>[2x]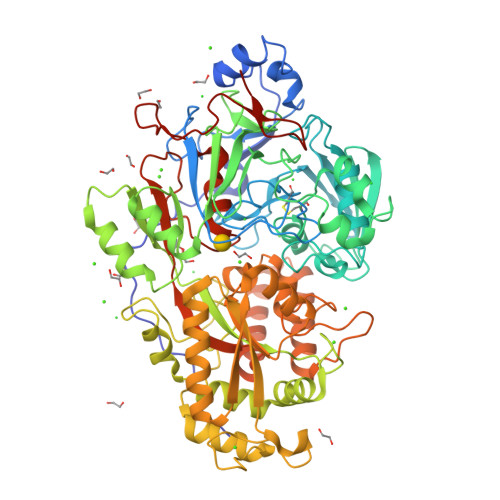MIALSANAFETTTPPEPPQFPAEGKINYVARDTILEFKALPSYSEPDWITEKFEKAGKLPPLKERLPEEPLVYKTGNMPDGVGVYGDTMRHVVGGRPEGWNYIAGQSQGWGGIDIALSECLTRTAPLFQVDAKDTEPLPNLAKSWEWSEDGHTLTMHLVKGAKWSDGEAFNADDVMFYWEDAVVDPNVSPLGGGASPEAFGEGTTLKKIDDYTVEWTFKAAFPKQYLYTMAYPSFCPGPSHILKPQHPKYSKNTYNQFKNAFPPEYMNMPVMGAWVPVSYRPDDLIVLRRNPYYWKVDEKGQQLPYLNEVHYKLSTWADRDVQAVAGSGDFSNLEQPENFVASLKRAADPNAPARLAFGPRLIGYNLQMNFSANGWGNPDERGQAIRELNRNEVFRQAVTSALDRKAIGDSLVKGPFTAIYPGGISSGTSFYDRASTVYYPFNLEGAKAALASIGLKDTDGDGFLNFPKETLGGRNVEITLLVNNGYATDKSLAEGLVGQMAKLGLRVVIHSLDSNQRDAAHYGGQFDWLVRRNSTELSSVVQNTEQLAPVGPRTSWNHRSPEGKELDLMPFEKEMADIVRKFISSQDNAERADLMKQYQKVYTQNLYTIGLTEYPGALIVNKRFSNVPQGTPIFMFNWAEDAIIRERLWVAADKQGKYELFPQQLPGKPGEGGPINHHHHHH>[6x]SNAMSKITFKDIYIDGNKITEDSRKAIYLLPPQPLKYASNTWIYKTMPTMNQWLKDIEVQKKMHLNQSSYHLSFSFPANEKIDEVLLEKIRELGFQIGVLELYVIEAKALKELSRKRDVDIQLVSSNNINDYLHVYDAFARPFGDSYANMVKQHIYSSYNLDDIERLVAYVNHQPVGIV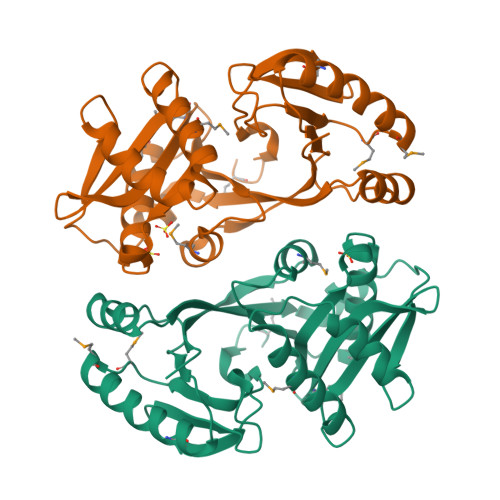DIIMTDKTIEIDGFGVLEEFQHQGIGSEIQAYVGRMANERPVILVADGKDTAKDMYLRQGYVYQGFKYHILKENI> MSYDVVIPAAGQGKRMKAGRNKLFIELKGDPVIIHTLRVFDSHRQCDKIILVINEQEREHFQQLLSDYPFQTSIELVAGGDERQHSVYKGLKAVKQEKIVLVHDGARPFIKHEQIDELIAEAEQTGAA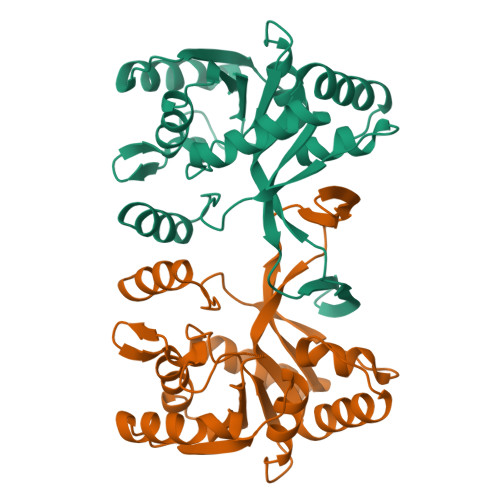ILAVPVKDTIKRVQDLQVSETIERSSLWAVQTPQAFRLSLLMKAHAEAERKGFLGTDDASLVEQMEGGSVRVVEGSYTNIKLTTPDDLTSAEAIMESESGNKHV> MSRSRPELGDWSSPAELAELQRSQLPRVLAQALRSPFYAARYRGTTPPRTADDFAGVEVTAKQDLRDQYPFGMLAVGREHLATYHESSGTAGEPTASYYTEEDWTDLAERFARKWTGIHPSDTFLVRTPYGLVITGHLAQAAGRLRGATVVPGDARSLATPLSRMVRVLKTLDVTLTWCNPTEITMLAAAAKAAGLRPDQDFPHLRAMFTAAEPLTEVRRRRLSEIWGGIPVVEEYGSTETGTIAGQCPEGRMHLWADRAIFEVYDPRTGTLSEAGRGQMVVTPLYRDAMPLLRYNLADDVEVSTDPCGCGWLLPTVTVLGRAGTGHRIGPATVTQQRLEELVFSLPAAYEVMFWRAKAHPDVLELEFEAPEPVRQRAVKELGAALDRELGVPHRITGLAPGTLVPAEALTAQRDI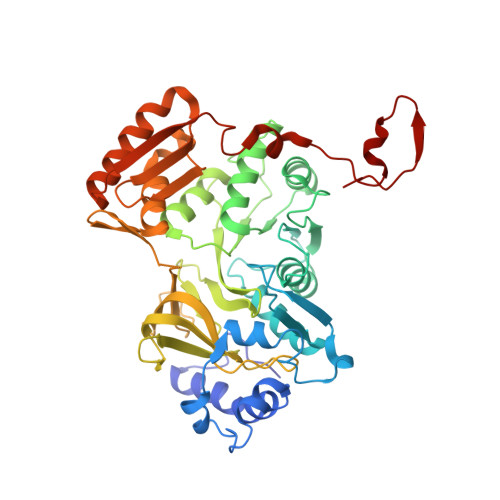LKARYLFAEDEDWDKAVMYF>AKSSYKLCVPAAYMKDCEQMLEVPTKSKVALECVPARDRVECLSFVQQRQADFVPVDPEDMYVASKIPNQDFVVFQEYRTDEEPDAPFRYEAVIVVHKDLPINNLDQLKGLRSCHTGVNRNVGYKIPLTMLMKRAVFPKMNDHSISPKENELKALSTFFAKSCIVGKWS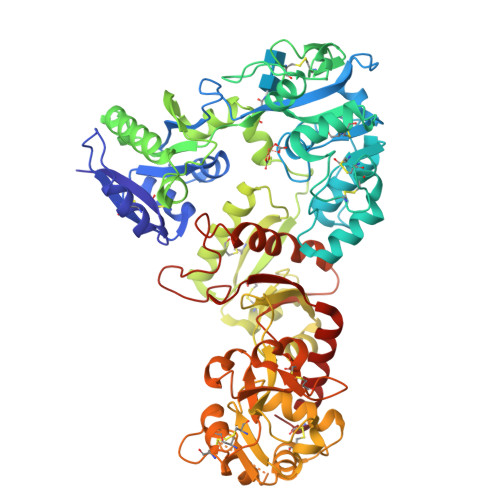PDPKTNSAWKSQYSHLCSMCEHPERCDYPDNYSGYEGALRCLAHNNGEVAFTKVIFTRKFFGLPVGTTPASPSNENPEEFRYLCVDGSKAPITGKACSWAARPWQGLIGHNDVLAKLAPLREKVKQLADSGAADKPEWFTKVLGLSEKIHHVADNIPIKPIDYLNKANYTEVIERGHGAPELVVRLCVTSNVALSKCRAMSVFAFSRDIRPILDCVQENSEDACLKSVQDNGSDLASVDDMRVAAAAKKYNLHPVFHEVYGELKTPNYAVAVVKKGTAYNKIDDLRGKKSCHSSYSTFSGLHAPLFYLINKRAIQSDHCVKNLGEFFSGGSCLPGVDKPENNPSGDDVSKLKKQCGSDSSAWKCLEEDRGDVAFVSSADLSHFDANQYELLCLNRDAGGRDVLSSFATCNVAMAPSRTWVAAKDFLSDVSIAHTPLSLAQMLATRPDLFNIYGEFLKNNNVIFNNAAKGLATTEKLDFEKFKTIHDVISSCGLA[2x]4-[(6-chloro-1-oxo-4-phenyl-3-propanoylisoquinolin-2(1H)-yl)methyl]benzoic 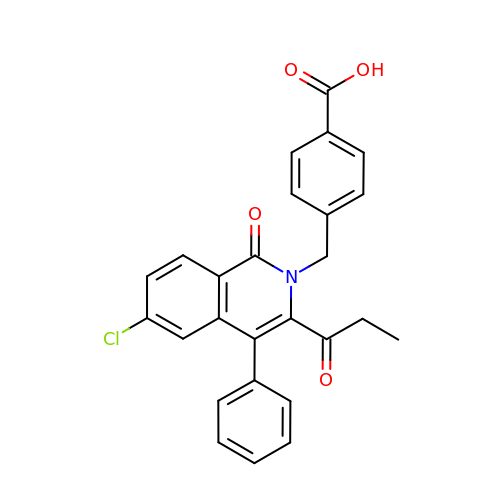acid | C26 H20 Cl N O4 | ITAZALHTZBIKDO-UHFFFAOYSA-N> MGNGPPMERAVSSDDILTYYNTFIFFIYFNFTNENIYIIYTIYMKVQNTIVYIVLLLIVV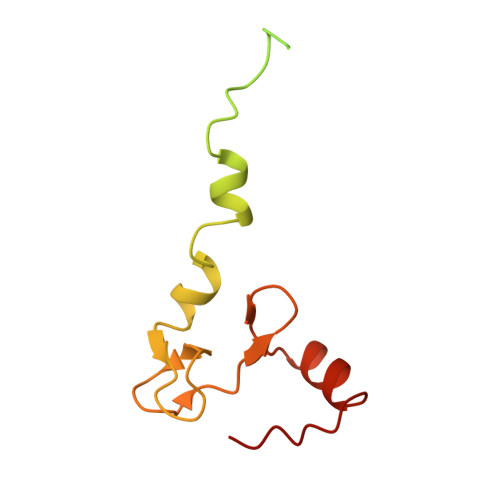VIIWNFTRKEGWSDYNAPNDFMKIYYSNIVEDKKLAEKYPFFGTGPFTGLRCRKPNNVGCNTTWVSGQLVELTPKLKEQIECKFGIQYVKT5-CHLORO-N-{(3S)-1-[(1S)-1-METHYL-2-MORPHOLIN-4-YL-2-OXOETHYL]-2-OXOPYRROLIDIN-3-YL}-1-BENZOTHIOPHENE-2-SULFONAMIDE | C19 H22 Cl N3 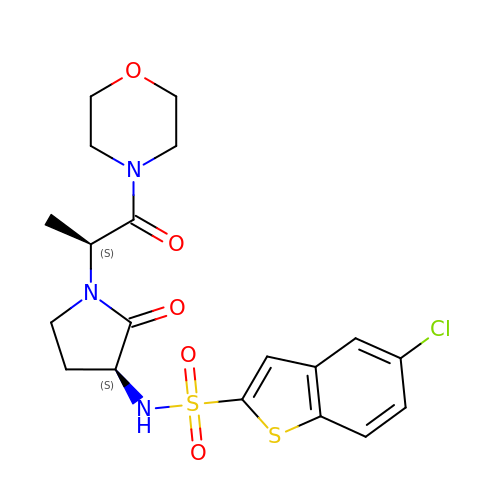O5 S2 | LTJNKFUIOOJXNJ-WFASDCNBSA-N> APLLESQRSNSEEKANFCSTHNDEVYARFRLQMRVGVRHSPLYTPSNMCMLDIEDSVEDIEESTEKEYASTATGEAAGVNVSVALVGEGVSIPFSYIGLGFNPSLEDSYLYVNVSSRAPWVKQTSDLSANGGWGIKQVLEKELLAIQ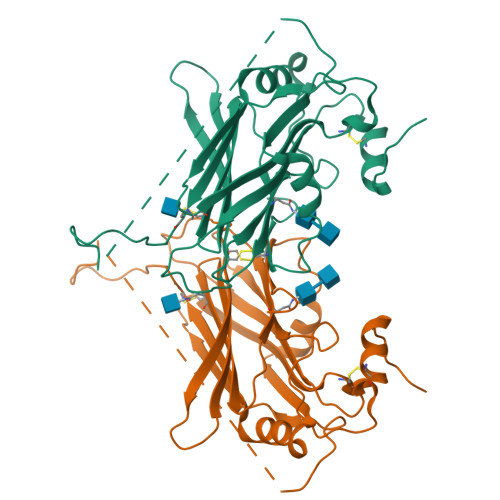IGCDNQKFPEEPTTTPPSPVTTTLSSTTPDLNEENTENTPTTTGASVDRKRNPADIDFSLLVDPRCVTSVDLHVELRDACIDYKQESPLSLKGKYGDGELVKKEIKDVGKNHNMCSLNLNPGN Miltiradiene | C20 H32 | 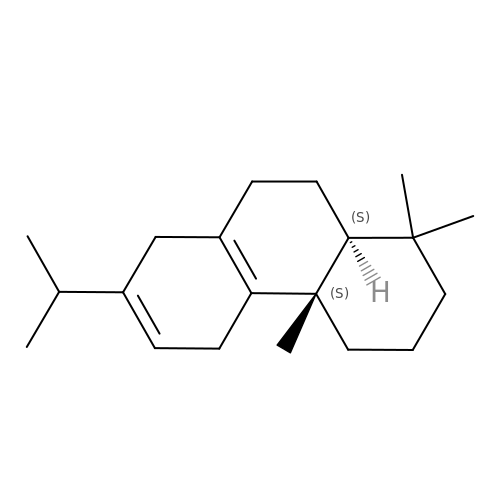BGVUIJDZTQIJIO-AZUAARDMSA-N> SMTTSKLEKTGLHVHEKIKHMVKNYGTMITGIPAEILGQNEAEISVGYVKKMGNMKENIAEVVRKSEMTQPTNSCGKASNEVCDLLLGTEGASEFEKSSYQVLSGDGSNLKGSLPNKNLLVRVEMDRFNAPQKYQKIKREEFNPETAEKNKIYLLEDQLV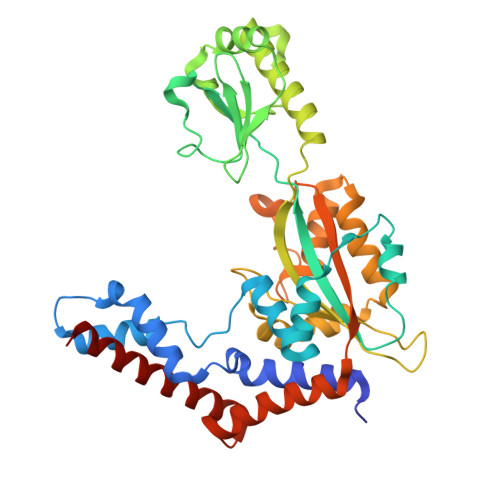YLDIFGKVIDLGQTSDTCHRLFNAITTPFYQNYILYDEYIDPEESAEEAAMFEMGEIVKAKMKNIDCWTATHSFTIFVPESDSEDTRTLYPYQAYWTSHTLQQWFSGDKDEKLSRLGIDGYIEKLALLGTTTDSKIRSSIYGELFSPPGKEHVFCTGMNEKFSPLRVKFKVTEVNPEIALQNLEEVQEFIDTNYPGENAKDQCELYKIKAQEAMTKQLEMRLLIEP> MLRESFAISGDSLISLASTGKRVPIKDLLGEKDFEIWAINEQTMKLESAKVSRVFCTGK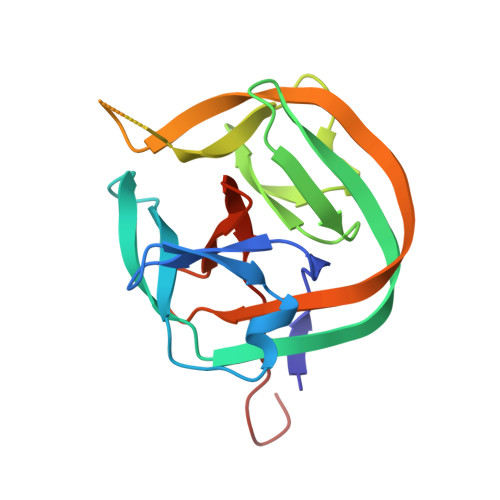KLVYTLKTRLGRTIKATANARFLTIDGWKRLDELSLKEHIALPRKLESSSLQLAPEIEKLPQSDIYWDPIVSITETGVEEVFDLTVPGLRNFVANDIIVHASIEQDKLGG While most SAM riboswitches strongly discriminate between SAM and SAH, the SAM/SAH riboswitch responds to both ligands with similar apparent affinities. The riboswitch forms an H-type pseudoknot structure with coaxial alignment of the stem–loop helix (P1) and the pseudoknot helix (PK). An additional three base pairs form at the non-open end of P1, and the ligand is bound at the interface between the P1 extension and the PK helix. Binding SAM or SAH stabilizes the PK helix, so structuring the Shine–Dalgarno sequence, sequestering it and preventing initiation of translation (OFF state).

All retain the adenosine moiety, with variations in the methionine chain attached to the 5′ position. The adenosine sections are bound identically in all six complexes, with the same four hydrogen bonds between the RNA and ligand in each case. The differences lie in the methionine section of the molecules. The sulfur atom is 3.8 Å away from the nearest RNA atom, leaving enough space to accommodate the SAM methyl group without steric clash, and the open binding site will readily accommodate the trajectory of the chain with a planar thioether (SAH) or tetrahedral sulfonium (SAM). This is further illustrated by the structure with AMP bound, showing that the 5′ phosphate group can be accommodated in this position. 5-bromocytidine was included at nucleotide 10 within P1 to provide phasing information.

>[6x]GGUCACAACGGCUUCCUGGCGUGACC;>[6x]AUUGGAGCA DIDEHYDROASPARTATE | C4 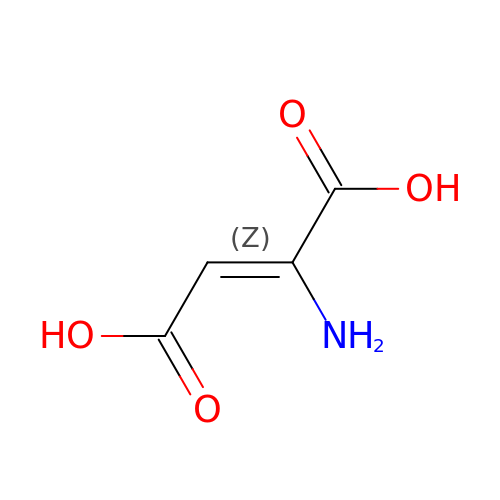H5 N O4 | ABZHGLSYGDUSDL-UPHRSURJSA-N> RICPRIWMECTRDSDCMAKCI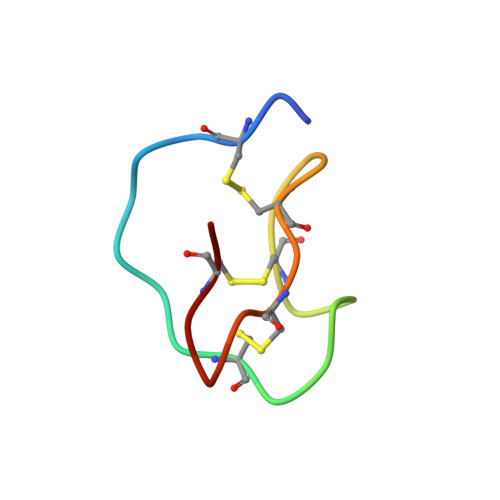CVAGHCG> KPRGKRGWLWLLLKLAIVFAVLIAIYGVYLDQKIRSRIDGKVWQLPAAVYGRMVNLEPDMTISKNEMVKLLEATQYRQVSKMTRPGEFTVQANSIEMIRRPFDFPDSKEGQVRARLTFDGDHLATIVNMENNRQFGFFRLDPRLITMISSPNGEQRLFVPRSGFPDLLVDTLLATEDRHFYEHDGISLYSIGRAVLANLTAGRTVQGASTLTQQLVKNLFLSSERSYWRKANEAYMALIMDARYSKDRILELYMNEVYLGQS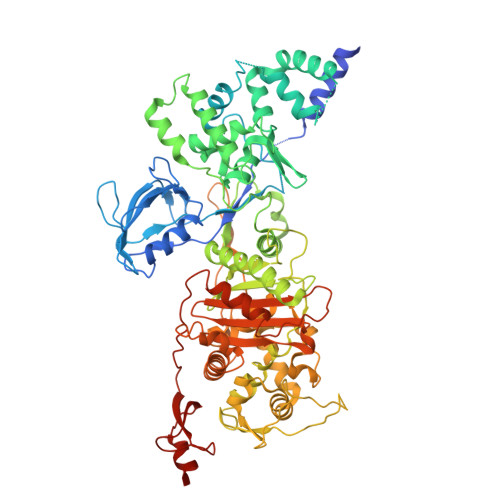GDNEIRGFPLASLYYFGRPVEELSLDQQALLVGMVKGASIYNPWRNPKLALERRNLVLRLLQQQQIIDQELYDMLSARPLGVQPRGGVISPQPAFMQLVRQELQAKLGDKVKDLSGVKIFTTFDSVAQDAAEKAAVEGIPALKKQRKLSDLETAIVVVDRFSGEVRAMVGGSEPQFAGYNRAMQARRSIGSLAKPATYLTALSQPKIYRLNTWIADAPIALRQPNGQVWSPQNDDRRYSESGRVMLVDALTRSMNVPTVNLGMALGLPAVTETWIKLGVPKDQLHPVPAMLLGALNLTPIEVAQAFQTIASGGNRAPLSALRSVIAEDGKVLYQSFPQAERAVPAQAAYLTLWTMQQVVQRGTGRQLGAKYPNLHLAGKTGTTNNNVDTWFAGIDGSTVTITWVGRDNNQPTKLYGASGAMSIYQRYLANQTPTPLNLVPPEDIADMGVDYDGNFVCSGGMRILPVWTSDPQSLCQQSEMQQQPS Rad18 interacts with the SMC5/6 localization factor 1 (SLF1) to recruit the SMC5/6 complex to DNA damage sites for repair. Previous studies have shown that the tandem BRCA1 C-Terminal (BRCT) domain repeat (tBRCT) at the SLF1 N-terminus (SLF1tBRCT) plays a critical role in the Rad18-SLF1 association. Our structure and biochemical studies demonstrate that SLF1tBRCT interacts with two phosphoserines and adjacent residues in Rad18 for high-affinity and specificity Rad18 recognition. We found that SLF1tBRCT utilizes mechanisms common among tBRCTs as well as unique ones for Rad18 binding, the latter include interactions with an α-helical structure in Rad18 that has not been observed in other tBRCT-bound ligand proteins.

Isothermal titration calorimetry (ITC) experiments indicated that SLF1tBRCT interacts strongly with a Rad18 peptide containing phosphorylated Ser442 and Ser444 (Rad18-2P), with a KD of 15 nM. The strong and specific Rad18-2P-SLF1tBRCT interaction enabled us to crystalize their complex and determine the structure to a resolution of 1.75 Å. Two SLF1tBRCT molecules were found in the asymmetric unit. Rad18 residues 437 to 452 and 436 to 451 were fitted into these densities on SLF1tBRCT molecules 1 and 2, respectively, revealing mostly identical structures for the two Rad18-2P peptides. The Rad18 peptide N-terminal half including the phosphoserines adopts an extended conformation and interacts with BRCT 1, its C-terminal half forms an α-helix and interacts primarily with BRCT 2. The Rad18-2P-SLF1tBRCT interface is the largest among tBRCT-ligand peptide structures reported to date, burying 1600 Å2 of surface area. Our structure revealed that phosphoserines 442 and 444 (pS442 and pS444) in Rad18 form distinct interactions with SLF1tBRCT. The pS442 side chain is completely buried at the Rad18-SLF1 interface. Its phosphate group forms polar interactions with the SLF1 Thr13 and Lys56 side chains and the Gly14 main chain carbonyl. In contrast, the pS444 side chain is mostly exposed to solvent. Its phosphate group forms polar interactions with the SLF1 Arg50 side chain in complex 2 in the crystal. The α-helix is stabilized by the pS444-Arg448 interaction and a Ser443-Asp449 hydrogen bond.

>[2x]MEDGTPKHIIQMTGFKMEEKEALVKLLLKLDCTFIKSEKYKNCTHLIAERLCKSEKFLAACAAGKWILTKDYIIHSAKSGRWLDETTYEWGYKIEKDSRYSPQMQSAPKRWREELKRTGAPGAFHRWKVVLLVRTDKRSDSLIRVLEAGKANVILPKSSPSGITHVIASNARIKAEKEKDNFKAPFYPIQYLGDFLLEKLEHHHHHH;>SDSCNSSSSDIIRDLLE[2x]>GPEFSMEDLIPLVNRLQDAFSAIGQNADLDLPQIAVVGGQSAGKSSVLENFVGRDFLPRGSGIVTRRPLVLQLVNATTEYAEFLHCKGKKFTDFEEVR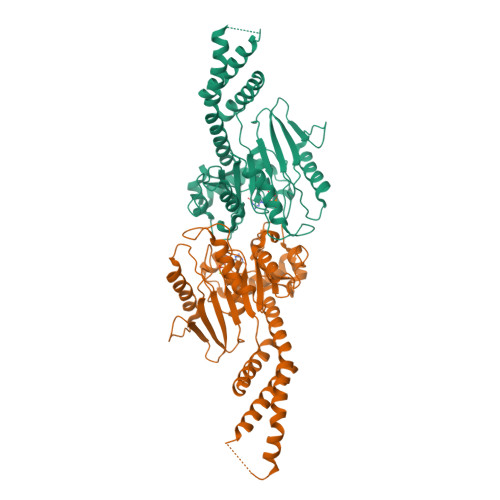LEIEAETDRVTGTNKGISPVPINLRVYSPHVLNLTLVDLPGMTKVPVGDQPPDIEFQIRDMLMQFVTKENCLILAVSPANSDLANSDALKVAKEVDPQGQRTIGVITKLDLMDEGTDARDVLENKLLPLRRGYIGVVNRSQKDIDGKKDITAALAAERKFFLSHPSYRHLADRMGTPYLQKVLNQQLTNHIRDTLPGLRNKLQSQLLSIEKEVEEYKNFRPDKHGTDSRVDEMLRMYHALKEALSIIGNINTTTV[2x]Here we present the crystal structure of the protein encoded by MGG_01005, a gene that is important for vegetative mycelial growth of M. oryzae. Although there is only low sequence conservation with the Dynein light chain Tctex-type 1 (dynlt1/3), from yeast, human, mouse and fruit fly, the crystal structure of the gene product, MGG_01005, adopts the dynein light-chain Tctex-1 fold. Pull-down and yeast two-hybrid analysis demonstrate an interaction with the N-terminal region of the M. oryzae dynein intermediate chain (DIC) MoDyn1I2 as observed for other dynlt1/3 proteins confirming MGG_01005 as the dynlt1/3 of M. oryzae. Importantly, the structure of a complex of MGG_01005 with an N-terminal peptide from MoDyn1I2117–150 together with mutagenesis studies reveal that a di-histidine motif, widely conserved in dynlt1/3 proteins interacts with a highly conserved glutamate residue in the DIC.

The 1.9 Å structure of the MGG_01005 was solved by single-wavelength anomalous diffraction (SAD). There is one protein molecule in the asymmetric unit (ASU) and the final refined model contains all residues except those between 80 and 112 that are not visible in the electron density map and are likely to be flexible or disordered. In addition, electron density for three extra residues (HHS) from the N-terminal His-tag is present. The monomer structure consists of two α helices (A to B) and 4 β-strands (β1-4). Three β-strands (β1-β3-β4) comprise an antiparallel β-sheet. The fourth strand β2, packs against the equivalent sheet (β1′-β3′-β4′) of a symmetry related molecule to form a dimer comprising an 8 stranded β-sandwich structure where each monomer has the topological arrangement αA-αB-β1-(β2′)-β3-β4, Fig. 1B. The configuration of this strand-swapped dimer and the magnitude of buried surface area: 1654 Å2 comprising 154 atoms from 43 residues in each molecule and a homodimer interface stabilized by 36 hydrogen bonds and 2 salt bridges suggests strongly that MGG_01005 is homodimeric in solution. This observation was confirmed by gel filtration chromatography and sedimentation velocity analytical ultracentrifugation measurements that demonstrate the dimer mass in solution. Among these interactions, Lys68 on β1 of one monomer (Monomer-A) interacts with Asp127′ on β3′ of the other monomer (Monomer-B) through two salt bridges. The rmsd and sequence similarity identity compared with Dm dynlt1/3 and Cm dynlt1/3 are 1.29 Å, 17.9% and 2.33 Å, 19.5% respectively.

> HHSMAAQGPSPIPTNRLKQIAADACNDAIGSAEFYDHAKTEQWNHQIINTILKAVIAESQPSDSTTPPQFKFAVNSTIVQHLVPSSKLNKPAGGADDKPASTATSTDGKPHVGRRGMHSATGAFWNDKTDGMWTYKHEGDESKGMDVVVMLIWIAV>[2x]QAGTTLTVDLSTTYQRIDGFGTSEAFQRAVQMSRLPEEGQRRALDVLFSTTNGAGLSILRNGIGSSPDMSSDHMVSIAPKSPGSPNNPLIYSWDGSDNKQLWVSQEAVHTYGVKTIYADAWSAPGYMKTNGNDANGGTLCGLSGAQCASGDWRQAYADYLT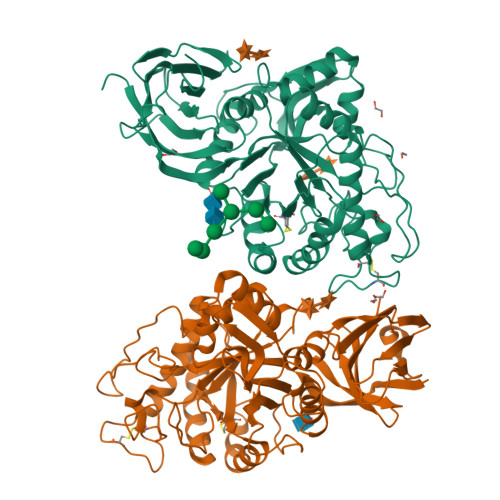KYVEFYQESNVTVTHLGFINAPELTTSYASMRFSASQAAEFIRILYPTIQKSNLTYKPTIACCDAEGWNSQAGMLGALSSVNSMFGLVTAHAYTSQPGFSMNTPHPVWMTAAADLQGAWTSAWYSYGGAGEGWTWANNVYNAIVNGNASAYLYWIGAQTGNTNSHMVHIDANAGTVEPSKRLWALGQWSRFVRPGARRVAVSGASGSLRTAAFRNEDGSVAVVVINSGGDAAVNVRLASSSSADQQPASAKAWATDNSRAIEEIQASFADGVATVNVPSRSMTTVVLYPAADAL>[2x]SWEE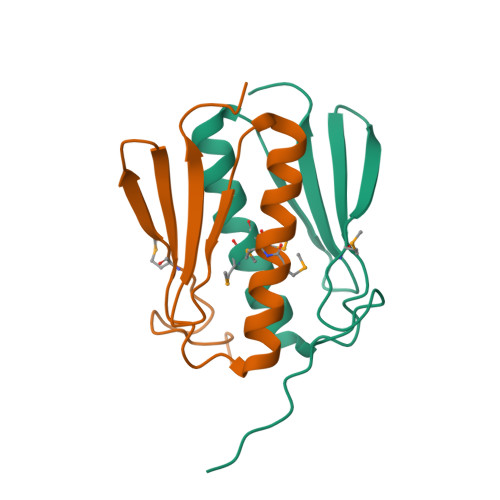ESTGIDLGFGPGIVMPSVSNHEGGTYVRYNGLGNVDPNYKNLISKMMRSLIGQIGNKYGYDIDLFDYQGDFLEVFLPHKPSK Icaridin | C12 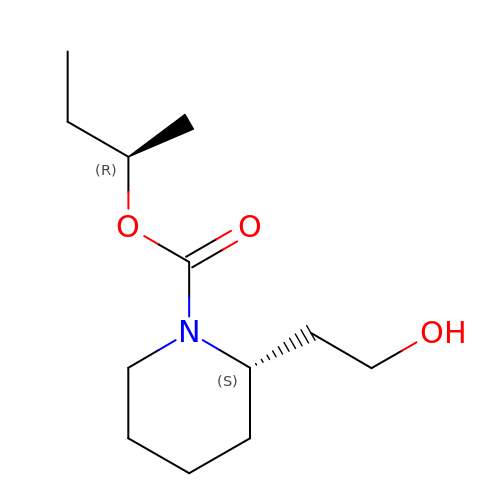H23 N O3 | QLHULAHOXSSASE-MNOVXSKESA-N Here, we present two crystal structures of GH73 enzymes from S. aureus, including glucosaminidase B (SagB) and the glucosaminidase part of major bifunctional autolysin (AtlA-gl). SagB crystallized with two and AtlA-gl with one molecule per asymmetric unit. In contrast to the crystal structure of AtlE and related N-acetylglucosaminidases, which were all observed in the closed form, these two proteins crystallized in the open form. Hence, for AtlA-gl and SagB to cleave a single glycan strand, both of their domains have to slide together into a closed conformation as observed in the AtlE structure.

AtlA-gl crystallized in the P6422 space group with one molecule per asymmetric unit. In spite of the weak diffraction data, its structure is well-resolved based on the electron density maps with the exception of the two N-terminal amino acid residues and the A128-N140 loop. The crystallographic R-factor of 0.29 reflects the irreproducible crystal, its small size and the low intensity of the diffraction data. Similar to SagB, the AtlA-gl structure also shares the topological layout of AtlE. Its R-domain comprises the region from A1 to D68 and A190 to K244, whereas the L-domain comprises from Q69 to K176. In contrast to the R-lobe, the L-lobe is smaller and partially disordered. The AtlA-gl structure was solved by molecular replacement using the SagB structure as the search model. The angle of rotation of the AtlA-gl structure superimposed on the R-domains and L-domains is 39° and resulted in a screw translational component of 4.6 Å. Thus, the packing of the R-domains and L-domains in the AtlA-gl structure differs from their packing in the AtlE structure even more than in the SagB structure. In the AtlA-gl structure, the 4th turn of helix α13 is stretched out compared to the slightly longer equivalent helix α15 in SagB and the even longer helix α12 in AtlE. The mutation of the tyrosine residue Y214 in the YATD region to alanine severely affected enzyme activity, whereas mutation of Y214 to phenylalanine completely restored the substrate degrading ability.

> AAELIKYNQTGMTLNQVAQIQAGLQYKPQVQRVPGKWTDANFNDVKHAMDTKRLAQDPALKYQFLRLDQPQNISIDKINQFLKGKGVLENQGAAFNKAAQMYGINEVYLISHALLETGNGTSQLAKGADVVNNKVVTNSNTKYHNVFGIAAYDNDPLREGIKYAKQAGWDTVSKAIVGGAKFIGNSYVKAGQNTLYKMRWNPAHPGTHQYATDVDWANINAKIIKGYYDKIGEVGKYFDIPQYK>GADSDDENSNFSSGITGMNLSAEVLKHQPMVEKYARENGISEYVNVLLAIIQVESGGTAEDVMQSSESLGLPPNSLDTESSIKQGCKYFASLLSSSKNQGIDDLNVAIQSYNYGGGYVGYVAGKGKKHTFNLAESFAREKSGGKKVTYTNPIAVAKNGGWRWNYGNMFYVE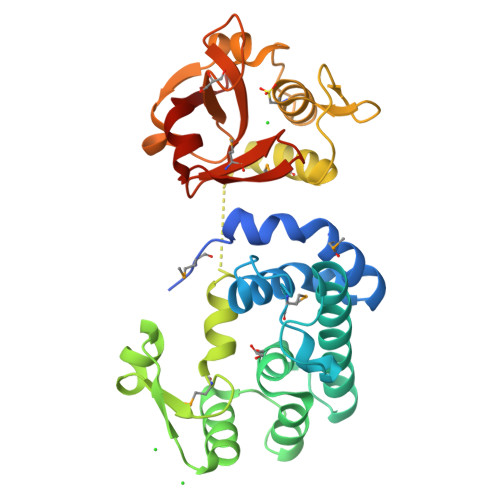LVNQYLTVPQVSGELAQKVMNEALKYQGWKYVYGGSNPNTSFDCSGLTQWCYGKAGISLPRTAQAQYDATQHLPLSQAKAGDLVFFHSTYNAGSYVTHVGIYVGNNQMYHAGDPIGYADLSSSYWQQHLIGAGRVKQ[6x]>ICYDAFVSYSERDAYWVENLMVQELENFNPPFKLCLHKRDFIPGKWIIDNIIDSIEKSHKTVFVLSENFVKSEWSKYELDFSHFRLFDENNDAAILILLEPIEKKAIPQRFCKLRKIMNTKTYLEWPMDEAQRE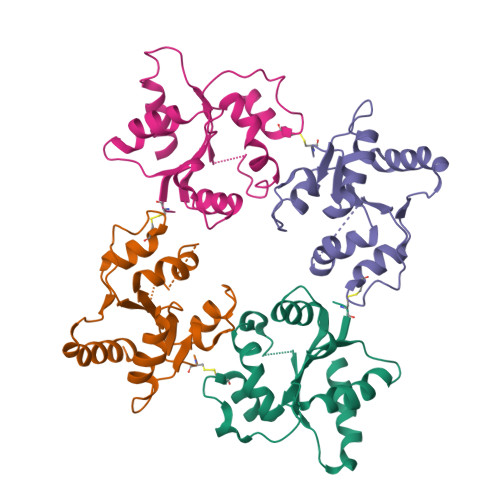GFWVNLRAAIKS[5x]>QPLGGESICSARAPAKYSITFTGKWSQTAFPKQYPLFRPPAQWSSLLGAAHSSDYSMWRKNQYVSNGLRDFAERGEAWALMKEIEAAGEALQSVHEVFSAPAVPSGTGQTSAELEVQRRHSLVSFVVRIVPSPDWFVGVDSLDLCDGDRWREQAALDLYPYDAGTDSGFTFSSP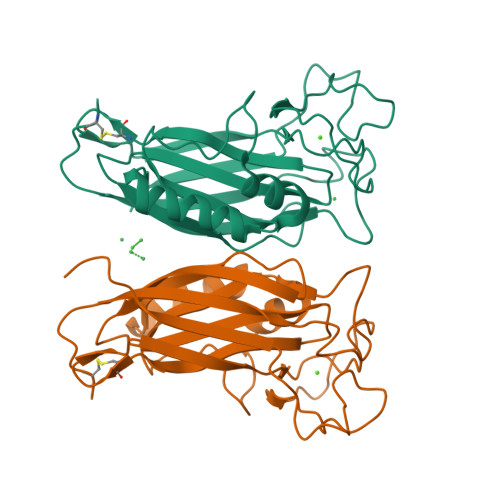NFATIPQDTVTEITSSSPSHPANSFYYPRLKALPPIARVTLLRLRQSPR[2x]>MVRVPLTAEELERGQRLGELLRSARGDMSMVTVAFDAGISVETLRKIETGRIATPAFFTIAAVARVLDLSLDDVAAVVTFGPVSTS[2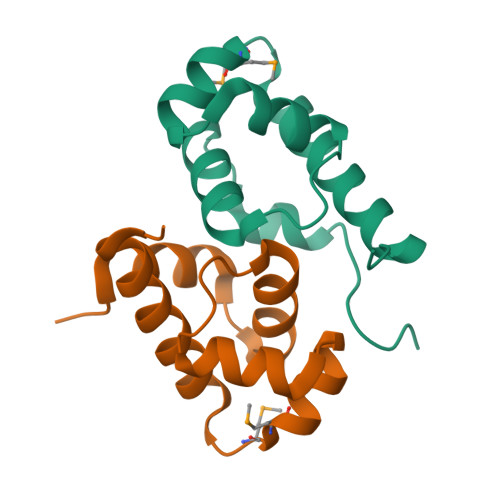x]>MSDIFNSPQNKASILTALMKSTTGDVEDVLIPKRFRPAKDPLDSPQAAAQFLKDNKYRILRPRAIPTMVELETDAALPRLRQMVEDGKLKDTVSVPEGTTAFYPKYYPFHKPDHDEVGTFGAPDITLLKQLTFFLLENDFPTGPETLRQVREAIATLQYGSGSYSGQLNRLLAMKGVATGRNPNKTPKTVGYTNEQLAKLLEQTLPINTPKHEDPDLRWAPSWLINYTGDLSTDKSYLPHVTIKSSAGLPYIGKTKGDTTAEALVLADSFIRDLGRAATSADPEAGVKKTITDFWYLSCGLLFPKGERYTQVDWDKKTRNIWSAPYPTHLLLSMVSTPVMNESKLNITNTQTPSLYGFSPFHGGMDRIMTIIRDSLDNDEDLVMIYADNIYILQDNTWYSIDLEKGEANCTPQHMQAMMYYLLTRGWTNEDGSPRYNPTWATFAMNVAPSMVVDSSCLLMNLQLKTYGQGSGNAFTFLNNHLMSTIVVAEWVKAGKPNPMTKEFMDLEEKTGINFKIERELKNLRETIVEAVETAPQDGYLADGSDLPPIRPGKAVELDLLGWSAIYSR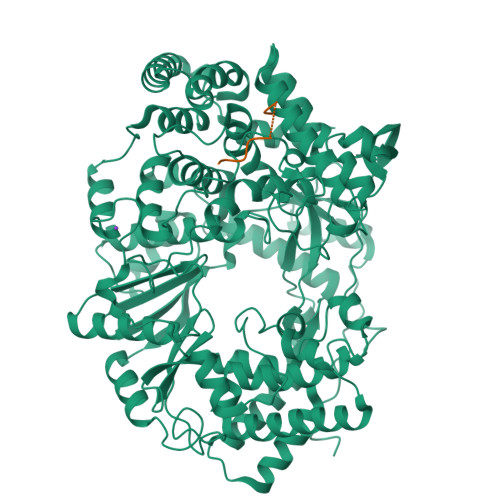QMEMFVPVLENERLIASAAYPKGLENKALARKPGAEIAYQIVRYEAIRLVGGWNNPLLETAAKHMSLDKRKRLEVKGIDVTGFLDDWNNMSEFGGDLEGITLSEPLTNQTLVDINTPLDSFDPKARPQTPRSPKKTLDEVTTAITSGTYKDPKSAVWRLLDQRTKLRVSTLRDQALALKPASSSVDNWAEATEELAQQQQLLMKANNLLKSSLTETREALETIQSDKIIAGKSNPEKNPGTAANPVVGYGEFSEKIPLTPTQKKNAKRREKQRRNQVEHHHHHH[3x];>GPTASGMDAELQGLLQATMARAKEVKDAEVFKLLKLMSWTRKNDLTDHMYEWSKEDPDAIKFGRLVSTPPKHQEKPKGPDQHTAQEAKATRISLDAVKAGADFASPEWIAENNYRGPSPGQFKYYMITGRVPNPGEEYEDYVRKPITRPTDMDKIRRLANSVYGLPHQEPAPDDFYQAVVEVFAENGGRGPDQDQMQDLRDLARQMKRRPRPAETRRQTKTPPRAATSSGSRFTPSGDDGEV[3x]> QDLARIEQFLDALWLEKNLAENTLNAYRRDLSMMVEWLHHRGLTLATAQSDDLQALLAERLEGGYK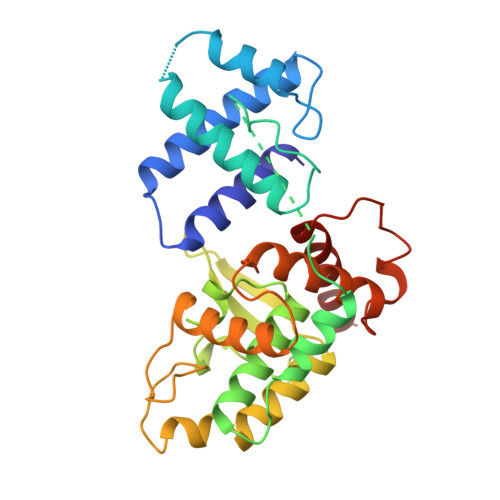ATSSARLLSAVRRLFQYLYREKFREDDPSAHLASPKLPQRLPKDLSEAQVERLLQAPLIDQPLELRDKAMLEVLYATGLRVSELVGLTMSDISLRQGVVRVIGKGNKERLVPLGEEAVYWLETYLEHGRPWLLNGVSIDVLFPSQRAQQMTRQTFWHRIKHYAVLAGIDSEKLSPHVLRHAFATHLLNHGADLRVVQMLLGHSDLSTTQIYTHVATERLRQLHQ>MVEIILSHLIFDQAYFSKVWPYMDSEYFESGPAKNTFKLIKSHVNEYHSVPSINALNVALENSSFTETEYSGVKTLISKLADSPEDHSWLVKETEKYVQQRAMFNATSKIIEIQTNAELPPEKRNKKMPDVGAIPDIMRQALSISFDSYVGHDWMDDYEARWLSYMNKARKVPFKLRILNKITKGGAETGTLNVLMAGVNVGKSLGLCSLAADYLQLGHNVLYISMEMAEEVCAKRIDANMLDVSLDDIDDGHISYAEYKGKMEKWREKSTLGRLIVKQYPTGGADANTFRSLLNELKLKKNFVPTIIIVDYLGICKSCRIRVYSENSYTTVKAIAEELRALAVETETVLWTAAQVGKQAWDSSDVNMSDIAESAGLPATADFMLAVIETEELAAAEQQLIKQIKSRYGDKNKWNKFLMGVQKGNQKWVEIE[6x]

The T4 bacteriophage gp41 helicase and gp61 primase assemble into a primosome to couple DNA unwinding with RNA primer synthesis for DNA replication. The domain architecture of the gp41 helicase resembles the bacterial DnaB helicase13,14 with an NTD and a RecA-like CTD that are connected by a linking helix (LH). The gp61 primase is composed of an N-terminal ZBD and a C-terminal RPD that are linked by an 18-residue flexible loop. Here we report a series of cryo-EM structures of T4 primosome assembly intermediates.

From step 2, we derived two 3D maps of the gp41 helicase hexamer bound to the ssDNA template. One map (map 2-I at 3.5 Å resolution) showed the ssDNA template in the helicase central channel, but the helicase hexamer remained in the right-handed open spiral form. The second state of primosome assembly is represented by map 2-I at 3.5 Å resolution and map 3-I at 2.9 Å, each with the ssDNA template bound in the central channel but with the gp41 helicase remaining an open spiral. Initial binding of the ssDNA caused only minor changes to the open spiral structure making it slightly more compact with a narrower gap and less mobility in subunits A and F. These minimal conformational changes indicate that the DNA-free gp41 helicase is competent for loading onto ssDNA, although a gp59 helicase loader protein is necessary for efficient helicase loading in vivo. In the open spiral gp41 helicase, the ssDNA binds to five (subunits B-F) of the six helicase subunits and coils inside the right-handed C-tier spiral, as compared to the activated helicase ring in which the sixth subunit (subunit A) now joins the other five subunits to coordinate the ssDNA phosphate backbone. Therefore, the 10 nt of the ssDNA stabilized in the inactive open spiral is increased to a total of 12 nt stabilized in the active closed ring gp41 helicase. Interestingly, ssDNA binding in the helicase central channel does not immediately induce gate closure, suggesting that the ssDNA-bound open spiral is a metastable state and that there is an energy barrier between the open spiral and the gate-closed, active ring configuration. Therefore, the gp41 helicase in the active closed-ring form, but not the inactive open-spiral form, can recruit a primase.>[8x]GPSRATPARKQMDKPEWKRVPNSEEDVRKCFGPRSVSRNFGDSDLVQ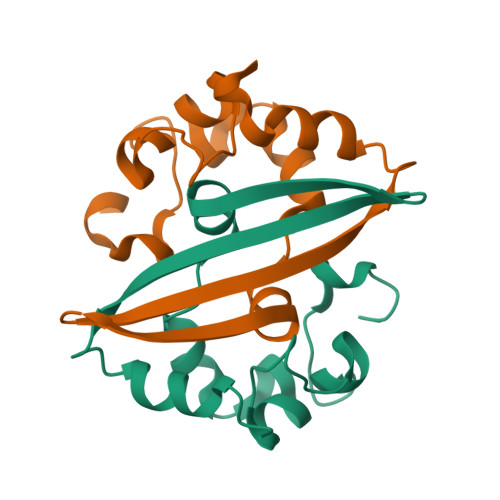HGVEAKHFPTIAELLPTQAALAFGSEITTKESGEFVEVTYHYVMKVPKTDKNLPRFLEQVSAYSK> ETGTSCPAACSCSNQASRVICTRRELAEVPASIPVNTRYLNLQENSIQVIRTDTFKHLRHLEILQLSKNLVRKIEVGAFNGLPSLNTLELFDNRLTTVPTQAFEYLSKLRELWLRNNPIESIPSYAFNRVPSLRRLDLGELKRLEYISEAAFEGLVNLRYLNLGMCNLKDIPNLTALVRLEELELSGNRLDLIRPGSFQGLTSLRKLWLMHAQVATIERNAFDDLKSLEELNLSHNNLMSLPHDLFTPLHRLERVHLNHNPWHCNCDVLWLSWWLKETVPSNTTCCARCHAPAGLKGRYIGELDQSHFTCYAPVIVEPPTDLNVTEGMAAELKC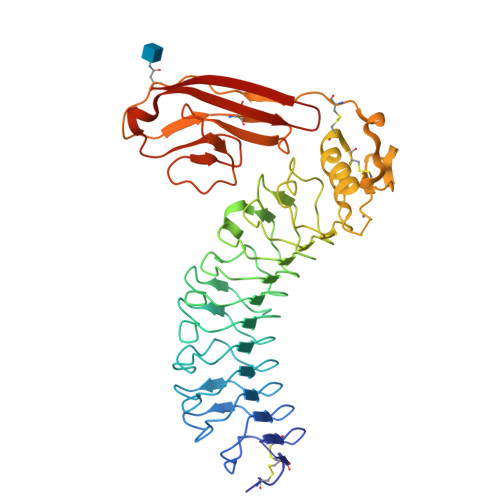RTGTSMTSVNWLTPNGTLMTHGSYRVRISVLHDGTLNFTNVTVQDTGQYTCMVTNSAGNTTASATLNVGTKHHHHHH>[4x]MRYAETGYVLEVDLTKGSIERVATDPRDTELYLGGLGTNAKILWDRVPPEVEPFSPENLLIFAAGLLCGTPATGCNRTIVSTVSPQTKLMAFSMMGGFWAPELKYAGYDKIIFRGKSPELVYLYINNDKVEIRDASHLKGKGAIETAEIIKKELNEPRAQVAAIGKAGENRVFYASIEQGRSSASRGGIGAVMGDKGLKAVVVRGTKDLCVAKPEEYIGLCNEVLDYIKHREENPIPDVMPILAGLGSPQEMKVHDEKWHTENFNWGNARTRRKDFWTDEVSHAWEKTMDKARTRLISCYNCPMKCGATISMEGLPTYMMKCFTKLTYTMAAYSDLDFGLRIAQKATEYGLDGFSAPQVMAFAFELLEKGILKDSDFPGLPEGNEERFFYLLDKIVNRDGIGDILANGTYWAAQEIGNGAEDYAHNNIKKHEQLPLKLSMLNPIYYLMYCTGEKINITQIEGQFPQAPYPKLEQR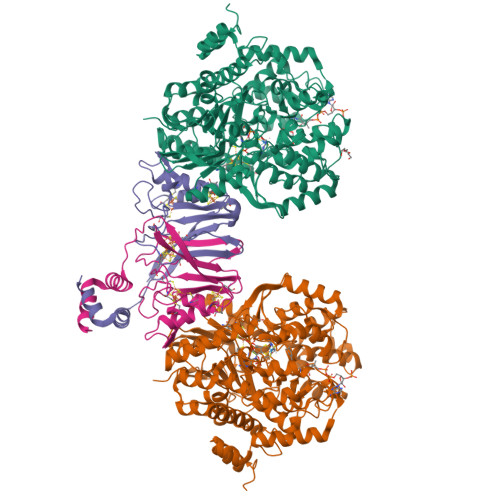EAFVEDWIQVPDEKFKKIFLEWEPRGEKSMPNFPTVDMCCDIVDWQEMMHYIDDALGQCAGLSSFPLKPPYHIHNYPKFIAAGAGIEMDTEKLKKAAKRYRTLVRAFNIRRGMRRVDEQPPANHWKNRFPELEKELLDSYYKLKGWNDDGIPTKETLDDLGLGYVGDEFIKRGILSAG;>MNSETKKRIVKTINIDADKCNGCRACEVICSAFHAMPPYSSNNPARSRVRVVRDPLRDIYVPLYAGEYTESECIGRDKFIIDGKEYDECGFCRASCPSRDLFREPDSGLPLKCDLCDGEPEPLCVKWCLVGALSVTEREVEEPDESVKRTEMEIGLESLISRFGADVVADTVEQLTKKR[4x]>PPFPWFGMDIGGTLVKLVYFEPKDITAEEEQEEVENLKSIRKYLTSNTAYGKTGIRDVHLELKNLTMCGRKGNLHFIRFPSCAMH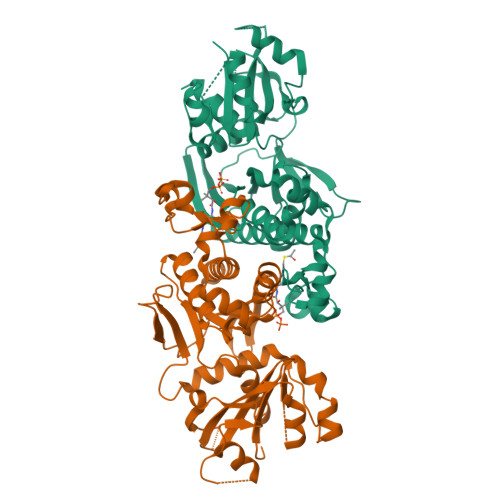RFIQMGSEKNFSSLHTTLCATGGGAFKFEEDFRMIADLQLHKLDELDCLIQGLLYVDSVGFNGKPECYYFENPTNPELCQKKPYCLDNPYPMLLVNMGSGVSILAVYSKDNYKRVTGTSLGGGTFLGLCCLLTGCETFEEALEMAAKGDSTNVDKLVKDIYGGDYERFGLQGSAVASSFGNMMSKEKRDSISKEDLARATLVTITNNIGSIARMCALNENIDRVVFVGNFLRINMVSMKLLAYAMDFWSKGQLKALFLEHEGYFGAVGALLELFK[2x]>[2x]MTVLEESADASSRRLAQRANGPATVLAIGTANPANVFEQSSYPDFYFDITNSQHMTELKLKFSRMCQKSGIKKRYMHLNSEILKANPSLCAYWEKSLDVRQDIAVVEVPKLGKEASLKAIKEWGQPKSKITHLVFCTTSGVDMPGADWALTKLLGLRP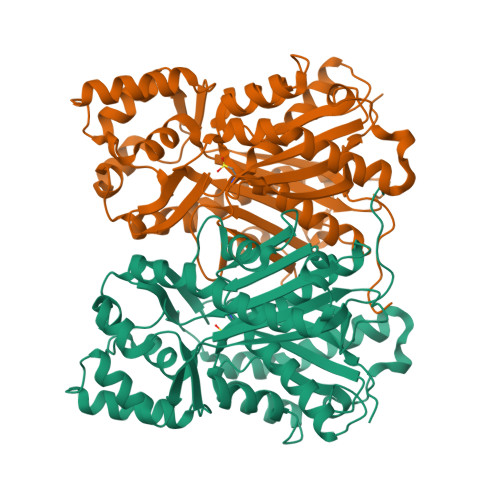SVKRLMMYQQGCFAGGTVLRVAKDVAENNKGARVLVVCSEITCVTFRGPSETHLDSLVGQALFGDGAAAVILGSDPLPEENPCFELHWSGSNILPDSDGAIDGHLREVGLTFHLMKDVPGIISKNIGKVLNDAFRSAFDESGNAEDRPASVNDIFWIAHPGGPAILDQVEEKMKLAPEKMRATRDVLSEYGNMSSACVLFIMDHMRRMSAQNKLQTTGEGLDWGVLLGFGPGLTVETVLLKSIRLAC> MINAIRTPDQRFS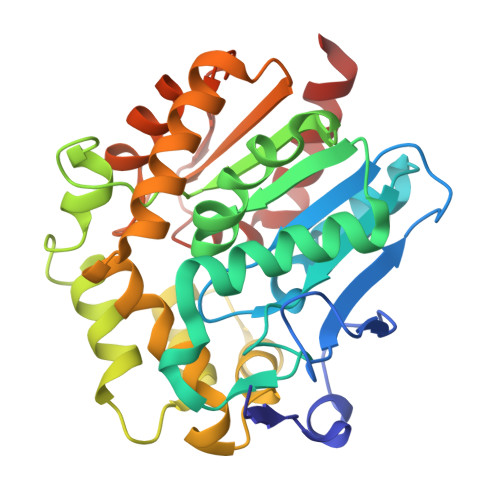NLDQYPFSPNYLDDLPGYPGLRAHYLDEGNSDAEDVFLCLHGEPTWSYLYRKMIPVFAESGARVIAPDFFGFGKSDKPVDEEDYTFEFHRNFLLALIERLDLRNITLVVQDWGGFLGLTLPMADPSRFKRLIIMNACLMTDPVTQPAFSAFVTQPADGFTAWKYDLVTPSDLRLDQFMKRWAPTLTEAEASAYAAPFPDTSYQAGVRKFPKMVAQRDQACIDISTEAISFWQNDWNGQTFMAIGMKDKLLGPDVMYPMKALINGCPEPLEIADAGHFVQEFGEQVAREALKHFAETE> MEHVAFGSEDIE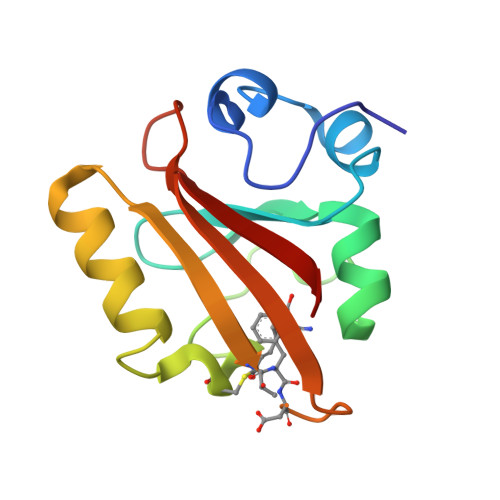NTLAKMDDGQLDGLAFGAIQLDGDGNILQYNAAEGDTTGRDPKQVIGKNFFKDVAPCTDSPEFYGKFKEGVASGNLNTMFEYTXDYQMTPTKVKVHMKKALSGDSYWVFVKRV>MSGKAPGSEGGSAPDGALTLGFAQVGAESGWRTANTESIKSAAEEAGVNLKFADANGEQEKQISAIRSFIQQGVDVIAFSPVVRTGWDAVLQETKNAGIPVILTDRAVDTQDTDVYKTFIGADFIEEGRRAGQWVADQYASATGPVNIVQLEGTTGADPAIDRKTGFAEGISKNPNLKIVASQTGDFTRSGGKQVMEAFLKSTPQIDVVFAQNDDMGLGAMEAIEAAGKKPGTDIKIVAVDATHDGMQALADGKFNYIVECNPL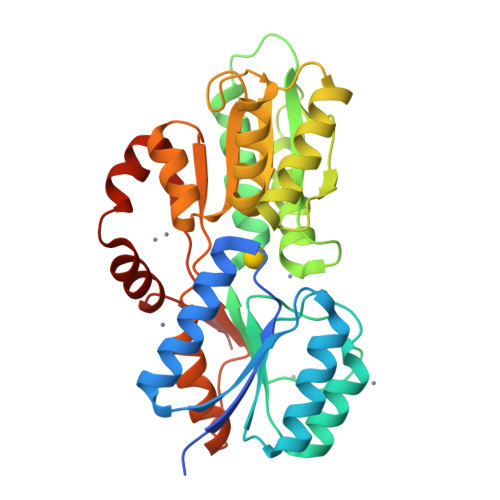LGPELMDLAKKVAAGEPVPERVVTPDEAFDQAQAKAALPNRQYKLAAALEHHHHHH[2x]> MKLKILDKDNATLNVFHRNKEHKTIDNVPTANLVDWYPLSNAYEYKLSRNGEYLELKRLRSTLPSSYGLDDNNQDIIRDNNHRCKIGYWYNPAVRKDNLKIIEKAKQYGLPIITEEYDANTVEQGFRDIGVIFQSLKTIVVTRYLEGKTEEELR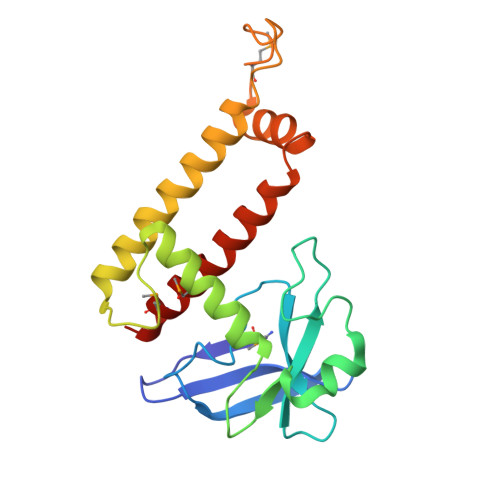IFNMKSEESQLNEALKESDFSVDLTYSDLGQIYNMLLLMKKISK>[2x]ATCYCRTGRCATHESLSGVC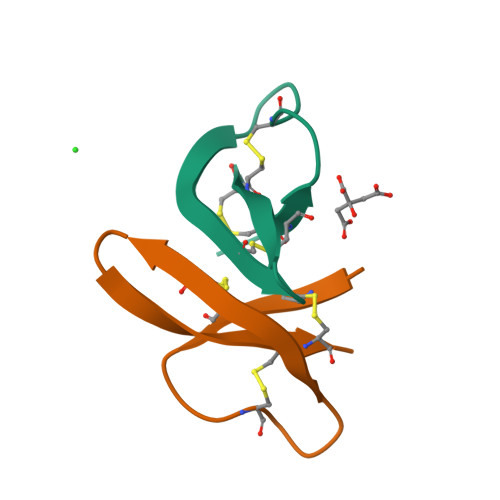EISGRLYRLCCR>MGKVNVAKLRYMSRDDFRVLTAVEMGMKNHEIVPGSLI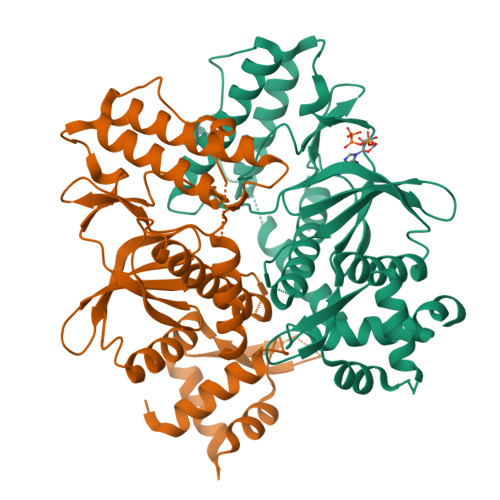ASIASLKHGGCNKVLRELVKHKLIAWERTKTVQGYRLTNAGYDYLALKTLSSRQVVESVGNQMGVGKESDIYIVANEEGQQFALKLHRLGRTSFRNLKNKRDYHKHRHNVSWLYLSRLSAMKEFAYMKALYERKFPVPKPIDYNRHAVVMELINGYPLCQIHHVEDPASVYDEAMELIVKLANHGLIHGDFNEFNLILDESDHITMIDFPQMVSTSHPNAEWYFDRDVKCIKDFFMKRFSYESELFPTFKDIRREDTLDVEVSASGYTKEMQADD[4x]> GPTSPGPALTDWARVREELASTGPPVVAM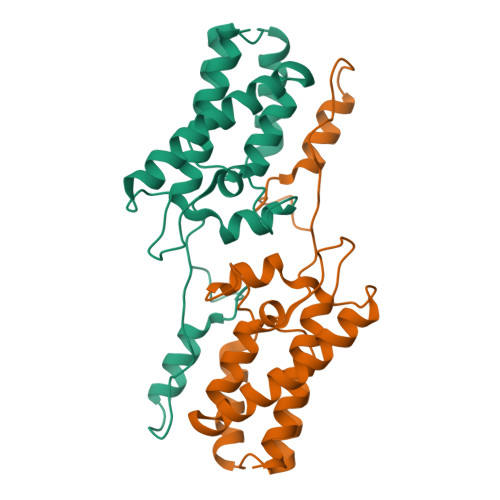PVVIKTEGPAWTPLEPKLITRLADTVRTKGLRSPITMAEVEALMSSPLLPHDVTNLMRVILGPAPYALWMDAWGVQLQTVIAAATRDPRHPANGQGRGERTNLNRLKGLADGMVGNPQGQAALLRPGELVAITASALQAFREVARLA>[4x]PGAPWWKSAVFYQVYPRSFKDTNGDGIGDFKGLTEKLDYLKGLGIDAIWINPHYASPNTDNGYDISDYREVMKEYGTMEDFDRLMAELKKRGMRLMVDVVINHSSDQHEWFKSSRASKDNPYRDYYFWRDGKDGHEPNNYPSFFGGSAWEKDPVTGQYYLHYFGRQQPDLNWDTPKLREELYAMLRFWLDKGVSGMRFATVATYSKTPGFPDLTPEQMKNFAEAYTQGPNLHRYLQEMHEKVFDHYDAVTAGEIFGAPLNQVPLFIDSRRKELDMAFTFDLIRYDRALDRWHTIPRTLADFRQTIDKVDAIAGEYGWNTFFLGNHDNPRAVSHFGDDRPQWREAS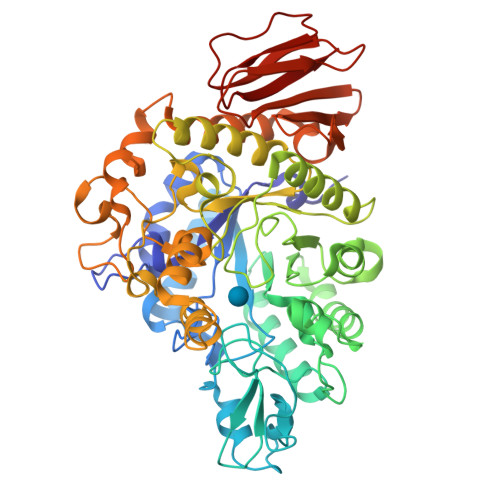AKALATVTLTQRGTPFIFQGDELGMTNYPFKTLQDFDDIEVKGFFQDYVETGKATAEELLTNVALTSRDNARTPFQWDDSANAGFTTGKPWLKVNPNYTEINAAREIGDPKSVYSFYRNLISIRHETPALSTGSYRDIDPSNADVYAYTRSQDGETYLVVVNFKAEPRSFTLPDGMHIAETLIESSSPAAPAAGAASLELQPWQSGIYKVK>[4x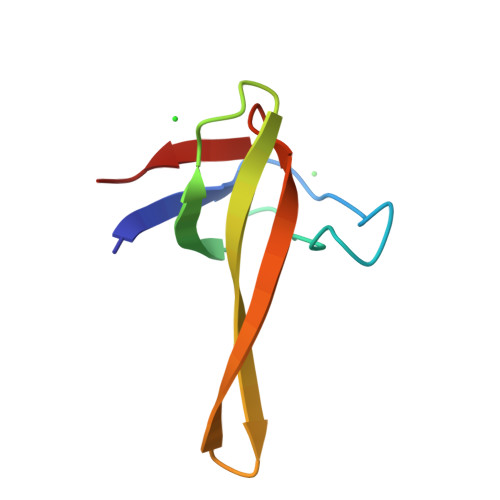]KELVLALYDYQEKSPREVTMKKGDILTLLNSTNKDWWKVEVKITVNGKTYERQGFVPAAYVKKLD> MTPLGPASSLPQSFLLKCLEQVRKIQGDGAALQEKLCATYKLCHPEELVLLGHSLGIPWAPLSSCPSQALQLAGCLSQLHSGLFLYQGLLQALEGISPELGPTLDTLQLDVADFATTIWQQMEELG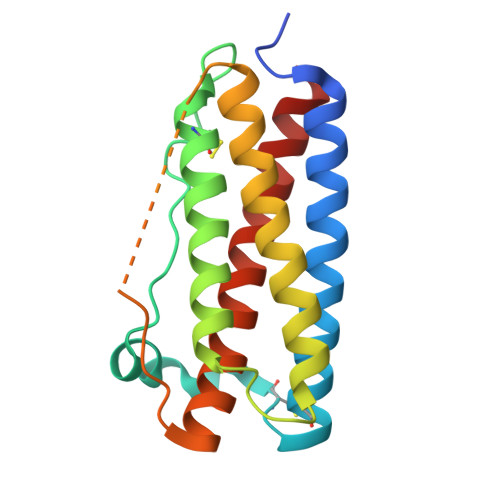MAPALQPTQGAMPAFASAFQRRAGGVLVASHLQSFLEVSYRVLRHLAQP>[2x]MLNNAMSVVILAAGKGTRMYSDLPKVLHTLAGKAMVQHVIDAANELGAAHVHLVYGHGGDLLKQALKDDNLNWVLQAEQLGTGHAMQQAA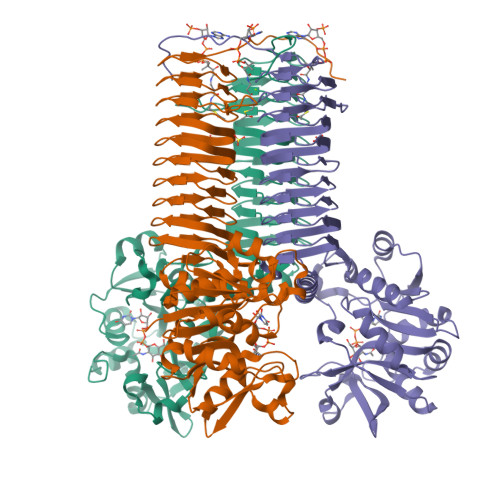PFFADDEDILMLYGDVPLISVETLQRLRDAKPQGGIGLLTVKLDDPTGYGRITRENGKVTGIVEHKDATDEQRQIQEINTGILIANGADMKRWLAKLTNNNAQGEYYITDIIALAYQEGREIVAVHPQRLSEVEGVNNRLQLSRLERVYQSEQAEKLLLAGVMLRDPARFDLRGTLTHGRDVEIDTNVIIEGNVTLGHRVKIGTGCVIKNSVIGDDCEISPYTVVEDANLAAACTIGPFARLRPGAELLEGAHVGNFVEMKKARLGKGSKAGHLTYLGDAEIGDNVNIGAGTITCNYDGANKFKTIIGDDVFVGSDTQLVAPVTVGKGATIAAGTTVTRNVGENALAISRVPQTQKEGWRRPVKKK>RMSDGAAPKANGSEASGQDLVPAAVEQAVPIQPVAGAALAAPAAGQINQIDPWIFQNFVQCPLGEFSISPRNTPGEILFDLALGPGLNPYLAHLSAMYTGWVGNMEVQLVLAGNAFTAGKVVVALVPPYFPKGSLTTAQITCFPHVMCDVRTLEPIQLPLLDVRRVLWHATQDQEESMRLVCMLYTPLRTNSPGDESFVVSGRLLSKPAADFNFVYLTPPIERTIYRMVDLPVIQPRLCTHARWPAPVYGLLV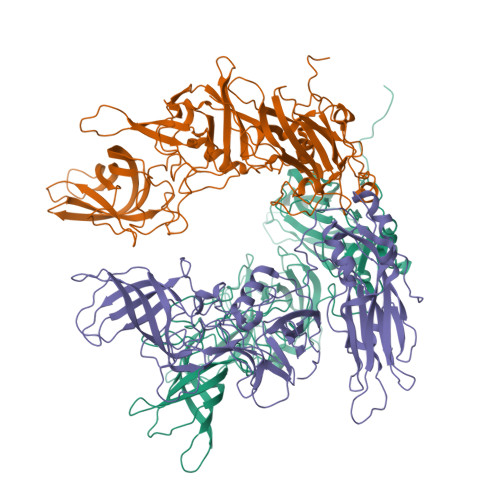DPSLPSNPQWQNGRVHVDGTLLGTTPISGSWVSCFAAEAAYEFQSGTGEVATFTLIEQDGSAYVPGDRAAPLGYPDFSGQLEIEVQTETTKTGEKLKVTTFEMILGPTTNADQAPYQGRVFASVTAAASLDLVDGRVRAVPRSIYGFQDTIPEYNDGLLVPLAPPIGPFLPGEVLLRFRTYMRQIDTADAAAEAIDCALPQEFVSWFASNAFTVQSEALLLRYRNTLTGQLLFECKLYNEGYIALSYSGSGPLTFPTDGIFEVVSWVPRLYQLASVGSLATGRMLKQ[3x]> SSGLVPRGSHMTAQTVTGAVAAAQLGATLPHEHVIFGYPGYAGDVTLGPFDHAAALASCTETARALLARGIQTVVDATPNDCGRNPAFLREVSEATGLQILCATGFYYEGEGATTYFK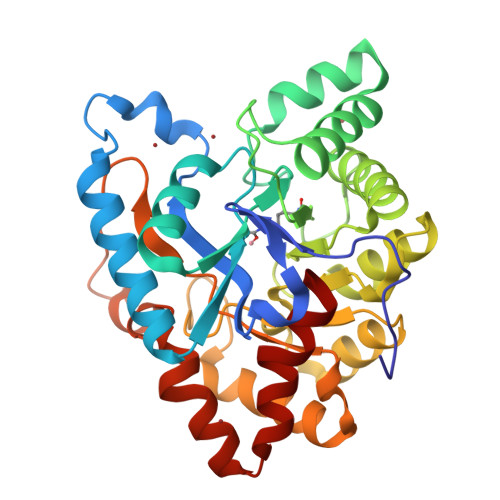FRASLGDAESEIYEMMRTEVTEGIAGTGIRAGVIKLASSRDAITPYEQLFFRAAARVQRETGVPIITHTQEGQQGPQQAELLTSLGADPARIMIGHMDGNTDPAYHRETLRHGVSIAFDRIGLQGMVGTPTDAERLSVLTTLLGEGYADRLLLSHDSIWHWLGRPPAIPEAALPAVKDWHPLHISDDILPDLRRRGITEEQVGQMTVGNPARLFG> MKIEEHHHHHHSSGRENLYFQGGAAQPAMAQGALLPAKAVYDFKAQTSKELSFKKGDTVYILRKIDQNWYEGEHHGR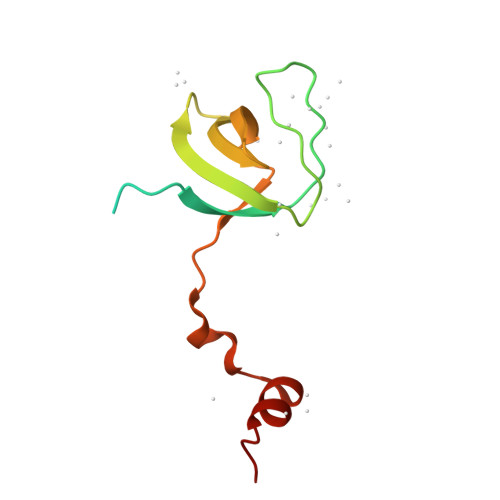VGIFPISYVEKLTGSAAALRTGEAYLRYVDAAA Based on sequence homology analyses, the bacterial SBP superfamily has been classified into 8 clusters, with cluster 5 comprising dipeptide binders (DppA family), oligopeptide binders (OppA family) and nickel specific SBP's (NikA family). Apart from GbpA and/or DppA representatives, some Pasteurellaceae also carry the genetic information for a close, although phylogenetically distinct homolog, which we have termed HbpA2 in the present paper. Interestingly, the HbpA2 clade diverged significantly from both the GbpA and DppA signature sequences. Because we were unable to identify a molecular interaction partner for these paralogous HbpA2 proteins, their in vivo role will have to await further study.

Indeed, our thermofluor analyses showed that none of the two HbpA2 proteins under study were able to interact with any of the tested type 5 SBP superfamily allocrites. The crystal structure of HbpA2Hp was determined to 2.0 Å resolution by maximum-likelihood molecular replacement. The structure reveals the two-lobe α/β-fold architecture and β-strand topology typical for SBP-like proteins, and is essentially identical to that of the structurally characterized GbpA and DppA proteins. Crystallographic refinement and exhaustive examination of residual difference electron density maps failed to provide any evidence for a bound ligand to HbpA2. Moreover, the N- and C-terminal domains were opened by about 33 degrees with respect to the GSSG-bound GbpA and glycylleucine-bound DppA reported previously, again indicating we crystallized apo-HbpA2Hp. Importantly, the crystal structure of HbpA2Hp offers an explanation for its inability to bind peptide-like ligands. Out of the 13 GSSG-contacting residues, 3 were not strictly conserved in HbpA2Hp, i.e. A380P, S430T, and D432R. Our structural analysis offers direct evidence that the A380P, S430T, and D432R substitutions would be grossly incompatible with GSH and GSSG binding as they would abolish electrostatic, H-bonding and hydrophobic interactions contributions critical for binding of such ligands. A similar analysis, this time against E. coli DppA, shows that R415 in HbpA2Hp takes the exact same position as the active site residue D408 in E. coli DppA, a residue that makes a salt-bridge with the amino-terminus of the bound dipeptide ligand. Thus, R415 would prevent dipeptide ligand binding.

> MDISAPTNTLVNCIATAPMKLSPAITNDANDFNASSQQVYNRLVEFKAGKIEVEPGLAERWEISEDGLVYTFYLRQNVKFHSNKTFSPTRPLNADDVVFSFQRQADKNHPYHNVSAGTYFYFNWMNLPSILKSVEKVDDYTVKITLNKPNTPFITTVAMDFLSIYSKEYADQLLAQGKPETLDQQPIGTGPFIFQTNQTDHAVRYTANVDYWKGKADIERLIFSITPDAGTRYAKLKAGECDVIDFPNISDIAQMKKDPQINLLEREGLNLAYIGLNTTKPELNNVKVRQALHHATDKKAIVDAVYQGGGTVATNPFPDAVLGYNPHLPQYEFNLEKAKALLAEAGYPNGFETEIWVQPVVRPSNPNPRRTAEIIQADWAKIGVKAKLVTHEWADFNKRTREGEFAAGTYGWTSRNGDPDNFLFPLFSQANIPGTNYSRWTDEKFEALLASAAQIQDTQTRAKLYQQAVEIFQQNSPIIPFAHSINYVPLNKRVQGFVQNPFGYTAFYGVSLKLEHHHHHH>[2x]SADQGEGRRDNNDVRNVNYRNPANDDMRNVNNRDNVDNNVNDNVNNNRVNDDNNNDRKLEVADEAADKVTDLKEVKHADIIVAGNQAYVAVVLTNGNKGAVENN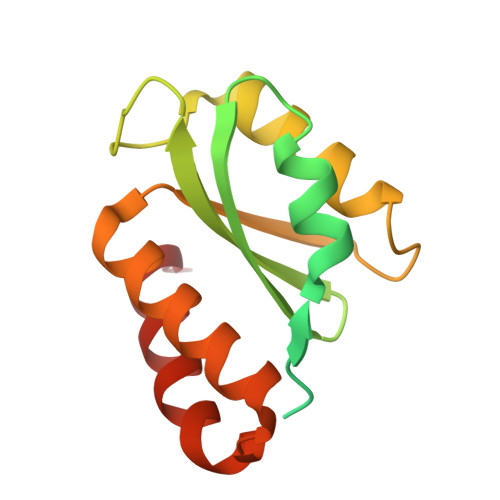LKKKIAKKVRSTDKNIDNVYVSANPDFVERMQGYGKRIQNGDPIAGLFDEFTQTVQRVFPNAE1-indol-1-ylethanone | C10 H11 N O | 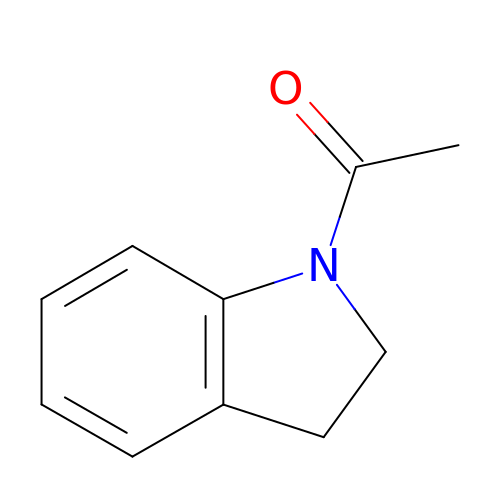RNTCWULFNYNFGI-UHFFFAOYSA-N>[2x]SKPKQPPDASPANLLTSLVRAHLDSGPS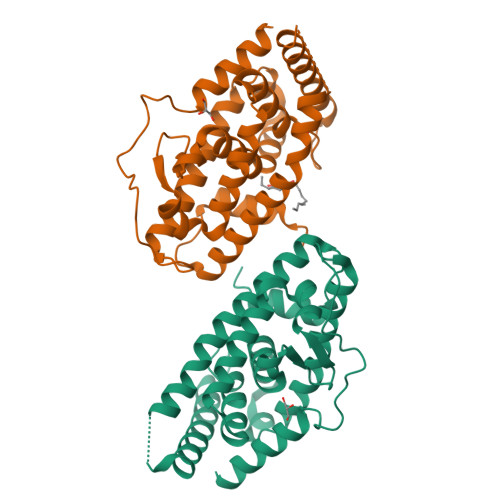TAKLDYSKFQELVLPHFGKEDAGDVQQFYDLLSGSLEVIRKWAEKIPGFAELSPADQDLLLESAFLELFILRLAYRSKPGEGKLIFCSGLVLHRLQCARGFGDWIDSILAFSRSLHSLLVDVPAFACLSALVLITDRHGLQEPRRVEELQNRIASCLKEHVAAVAGEPQPASCLSRLLGKLPELRTLCTQGLQRIFYLKLEDLVPPPPIIDKIFMDTLPFLEHHHHHH>GMASLKAKVLETFLAKSRPELLEYYIKVILDYNTAHNKVALSECYTVASVAEMPQNYRPHPQRFTYCSQVLGLHCYKKGIHYWEVELQKNNFCGVGICYGSMNRQGPESRLGRNSASWCVEWFNTKISAWHNNVEKTLPSTKATRVGVLLNCDHGFVIFFAVADKVHL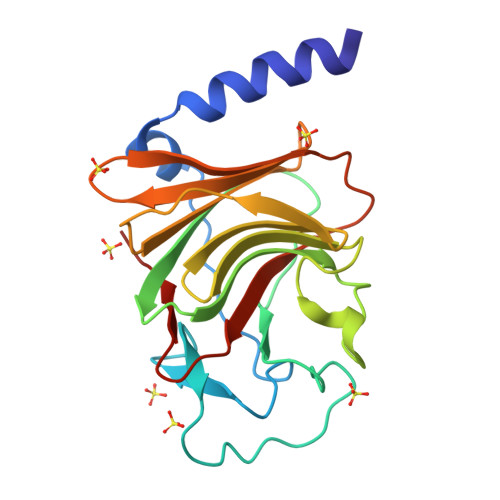MYKFRVDFTEALYPAFWVFSAGATLSICSPK[3x]>[4x]GSTLDVNQDSGTPFNPKEEIVVEKFLPTEGRKGTRVVVYGRNFGNDVSKVKVTIGGYPAKVINVKGESLLCICPSKAYEGDVKVSVVGDDEAELKSGVCEAKFDYQYNYVVTTFLGKLYENNTKWDVLAGPFDDCGAFDNIWRMMFDPNSN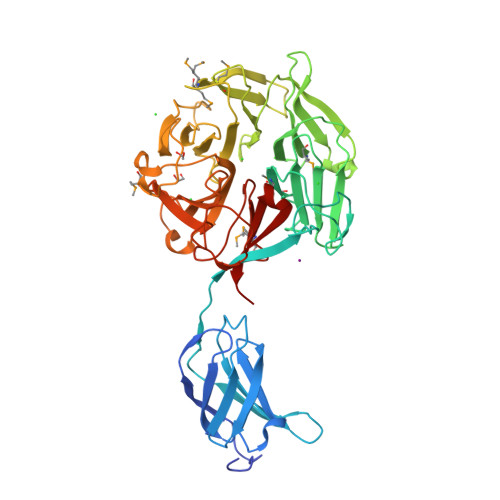YDDLYWVGQRDAFRHVDFVNQYVDIKTTNIGQCADVNFTLNGDMVVVDDQSSDTNTGIYLFTRASGFTERLSLCNARGAKTCAVHPQNGKIYYTRYHHAMISSYDPATGTLTEEEVMMDTKGSNFHIVWHPTGDWAYIIYNGKHCIYRVDYNRETGKLAVPYIVCGQHSSPGWVDGMGTGARLWGPNQGIFVKNEAYAGEEDEYDFYFCDRDSHTVRVLTPEGRVTTYAGRGNSREWGYVDGELRSQALFNHPTSIAYDMKRKCFYIGDCDNHRVRKIAPEE> YVATRDNCCILDERFGSYCPTTCGIADFLSTYQTKVDKDLQSLEDILHQVENKTSEVKQLIKA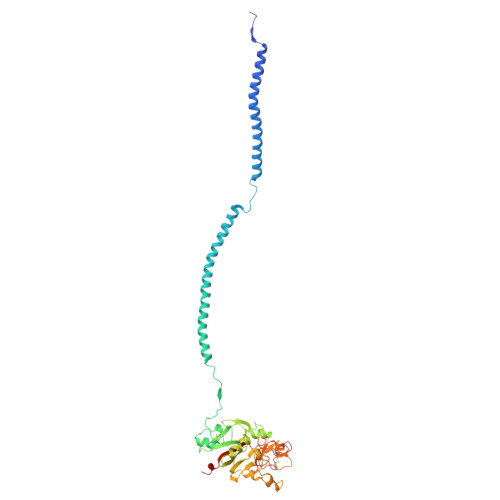IQLTYNPDESSKPNMIDAATLKSRKMLEEIMKYEASILTHDSSIRYLQEIYNSNNQKIVNLKEKVAQLEAQCQEPCKDTVQIHDITGKDCQDIANKGAKQSGLYFIKPLKANQQFLVYCEIDGSGNGWTVFQKRLDGSVDFKKNWIQYKEGFGHLSPTGTTEFWLGNEKIHLISTQSAIPYALRVELEDWNGRTSTADYAMFKVGPEADKYRLTYAYFAGGDAGDAFDGFDFGDDPSDKFFTSHNGMQFSTWDNDNDKFEGNCAEQDGSGWWMNKCHAGHLNGVYYQGGTYSKASTPNGYDNGIIWATWKTRWYSMKKTTMKIIPFNRLTIGEGQQHHLGGAKQAGDV>[2x]MIGYQIYVRSFRDGNLDGVGDFRGLKNAVSYLKELGIDFVWLMPVFSSISFHGYDVVDFYSFKAEYGS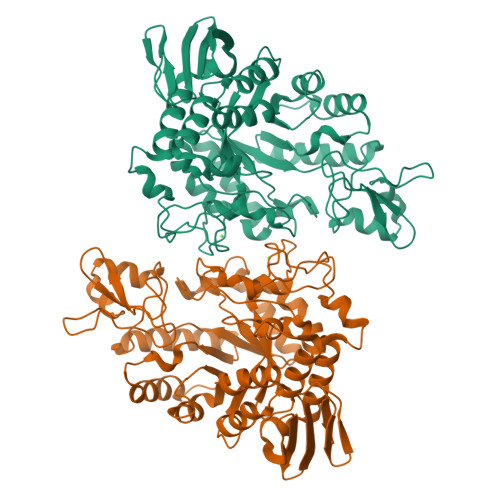EREFKEMIEAFHDSGIKVVLDLPIHHTGFLHTWFQKALKGDPHYRDYYVWANKETDLDERREWDGEKIWHPLEDGRFYRGLFGPFSPDLNYDNPQVFDEMKRLVLHLLDMGVDGFRFDAAKHMRDTIEQNVRFWKYFLSDLKGIFLAEIWAEARMVDEHGRIFGYMLNFDTSHCIKEAVWKENTRVLIESIERAVIAKDYLPVNFTSNHDMSRLASFEGGFSKEKIKLSISILFTLPGVPLVFYGDELGMKGVYQKPNTEVVLDPFPWNESMCVEGQTFWKWPAYNGPFSGISVEYQKRDPDSILSHTLGWTRFRKENQWIDRAKLEFLCKEDKFLVYRLYDDQHSLKVFHNLSGEEVVFEGVKMKPYKTEVV CITRYL-THIOETHER-COENZYME 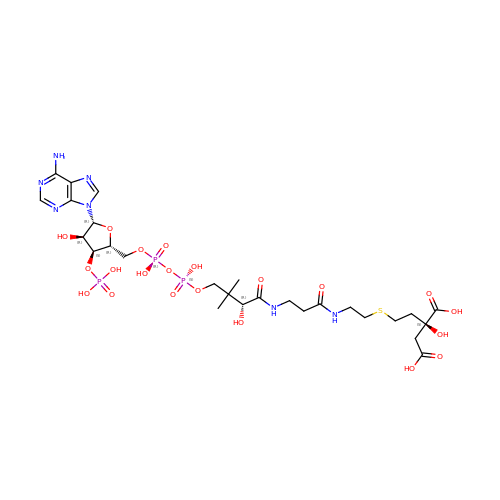*A | C27 H44 N7 O21 P3 S | VPFUWJMPUQBRCJ-QVYRMQCDSA-N>MPGSLIDTRQQPLSVGIVGGGIIGVILAAGLVRRGIDVKVFEQARGFREIGAGMAFTANAVRCMEMLDPAIVWALRSSGAVPISIGDHQAEARDYLRWVDGYHESSKRLYQLDAGIRGFEACRRDQFLEALVKVLPEGIVECQKRLQKIHEKNETEKVTLEFADGTFAHVDCVIGADGIRSRVRQHLFGEDSPYSHPHYSHKFAFRGLITMENAISALGEDKARTLNMHVGPNAHLIHYPVANETMVNIAAFVSDPEEWPDKLSLVGPATREEAMGYFANWNPGLRAVLGFMPENIDRWAMFDTYDYPAPFFSRGKICLVGDAAHAAVPHHGAGACIGIEDALCATVLLAEVFVSTRGKSSIVRNRAIAAAFGSFNAVRRVRAQWFVDSSRRVCDLYQQPEWADPQ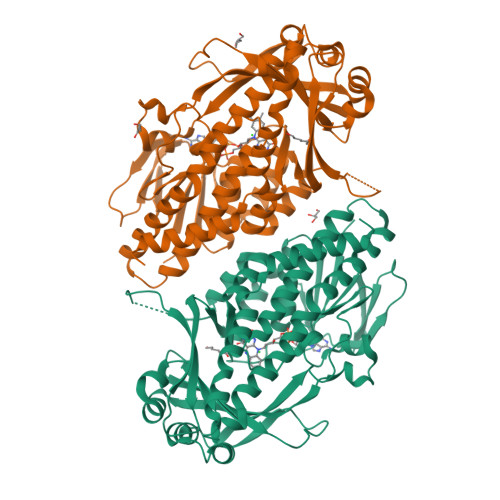KRIKAENCFEEIKDRSHKIWHFDYNSMLQEAIEKYRHNMGS[2x]>VTALSRLGEPPSGHDGNSEVRRIAMKRATVPVLRRVAAVCAAALLVTVGTGGPASATGTRSAICRATTVEVTLGKGTGKMWGELCRPAGSSPDTVVTMVHGATYNHNYWDFPYQPDKYSFRKMLNGAGYATFVVDRLGTGNSTVPPSSELNLTVEARQMHEVVQGLRTGRIGGTGFGKVVLAGYSLGSAVTSIEASTFHDVDAVLITALGHYNNPAGTQAIIDNGLSPNDDPVLKDRHHYDDGYATTKPGSRKHVFYADRPMDPGVLATDELTKDANVFTEAADPLVIDPAVSRAIDVPVMFALGDRDPLMCGDGYEDCSSQAALRAQEAPFWTSAPSFDVILVEDAGHGLNLVPNTRVYQDASRDW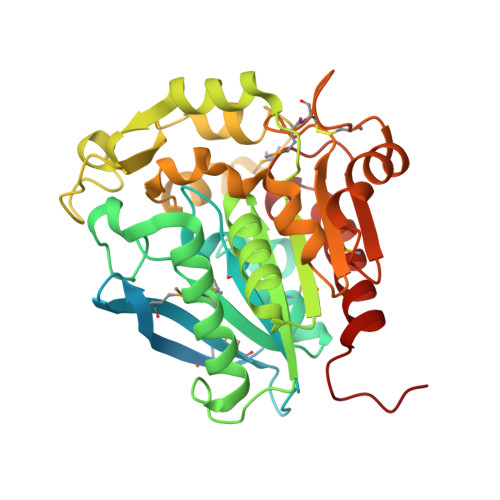LDRVVGHGLEHHHHHH[4x]dodecaphosphate | H14 O37 P12 | 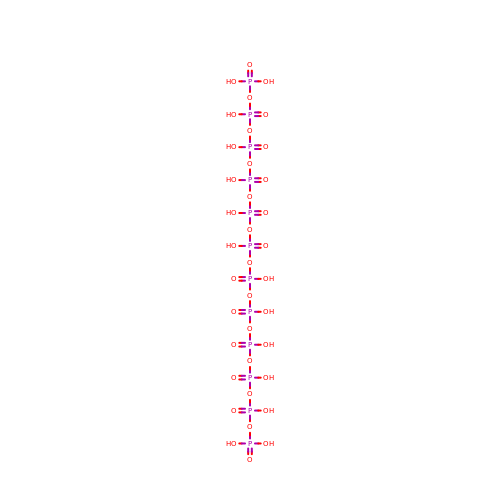NXLWQEGXNVMZEN-UHFFFAOYSA-N>[7x]MTMFQYYKRSRHFVFSAFIAFVFVLLCQNTAFARASSNGDLPTKADLQAQLDSLNKQKDLSAQDKLVQQDLTDTLATLDKIDRIKEETVQLRQKVAEAPEKMRQATAALTALSDVDNDEETRKILSTLSLRQLETRVAQALDDLQNAQNDLASYNSQLVSLQTQPERVQNAMYNASQQLQQIRSRLDGTDVGETALRPSQKVLMQAQQALLNAEIDQQRKSLEGNTVLQDTLQKQRDYVTANSARLEHQLQLLQEAVNSKRLTLTEKTAQEAVSPDEAARIQANPLVKQELEINQQLSQRLITATENGNQLMQQNIKVKNWLERALQSERNIKEQIAVLKGSLLLSRILYQQQQTLPSADELENMTNRIADLRLEQFEVNQQRDALFQSDAFVNKLEEGHTNEVNSEVHDALLQVVDMRRELLDQLNKQLGNQLMMAINLQINQQQLMSVSKNLKSILTQQIFWVNSNRPMDWDWIKAFPQSLKDEFKSMKITVNWQKAWPAVFIAFLAGLPLLLIAGLIHWRLGWLKAYQQKLASAVGSLRNDSQLNTPKAILIDLIRALPVCLIILAVGLILLTMQLNISELLWSFSKKLAIFWLVFGLCWKVLEKNGVAVRHFGMPEQQTSHWRRQIVRISLALLPIHFWSVVAELSPLHLMDDVLGQAMIFFNLLLIAFLVWPMCRESWRDKESHTMRLVTITVLSIIPIALMVLTATGYFYTTLRLAGRWIETVYLVIIWNLLYQTVLRGLSVAARRIAWRRALARRQNLVKEGAEGAEPPEEPTIALEQVNQQTLRITMLLMFALFGVMFWAIWSDLITVFSYLDSITLWHYNGTEAGAAVVKNVTMGSLLFAIIASMVAWALIRNLPGLLEVLVLSRLNMRQGASYAITTILNYIIIAVGAMTVFGSLGVSWDKLQWLAAALSVGLSFGLQEIFGNFVSGLIILFERPVRIGDTVTIGSFSGTVSKIRIRATTITDFDRKEVIIPNKAFVTERLINWSLTDTTTRLVIRLGVAYGSDLEKVRKVLLKAATEHPRVMHEPMPEVFFTAFGASTLDHELRLYVRELRDRSRTVDELNRTIDQLCRENDINIAFNQLEVHLHNEKGDEVTEVKRDYKGDDPTPAVG

Amongst these family members, MscK is unique in that channel activation, in addition to elevated lateral membrane tension, requires the presence of certain external ions such as K+, Rb+, or Cs+ 32–34. The E. coli MscK (EcMscK) channel, consisting of 1120 amino acids, contains a large N-terminal periplasmic domain (PD, ~500 amino acids), a transmembrane domain (TMD) with eleven predicted TM helices, and a cytoplasmic domain (CTD) analogous to that of EcMscS. The MscK channel forms a symmetric heptamer, with each subunit comprised of three distinct layers: an N-terminal periplasmic PD, a TMD with eleven TM helices, and a C-terminal cytoplasmic CTD. To better understand the biophysical underpinnings of mechanotransduction and to establish the molecular basis of dual activation in a ligand- and force-gated channel, we have determined cryo-EM structures of EcMscK in distinct functional states by leveraging GOF mutants.

To potentially improve structural homogeneity and to achieve a functionally distinct conformation, we decided to characterize a GOF mutant G924S, which, in contrast to the WT channel, was active under elevated membrane tension in both KCl and NaCl conditions. Thus, the cryo-EM datasets of G924S in NaCl and in KCl were essentially indistinguishable, which allowed us to combine the datasets to further improve the reconstructions of both the closed and open conformations to overall resolutions of 3.84 and 3.47 Å, respectively. The final atomic models fit well into their respective densities and were refined to good stereochemistry. The lower resolution reconstruction of the WT channel is nearly identical to the closed conformation of G924S, and hereinafter the higher-resolution structures of G924S are primarily used for structural analysis and interpretation. The innermost pore-lining helix TM11 contains an apparent kink such that TM11a defines the transmembrane ion-conduction path and TM11b runs nearly parallel to the membrane plane and extends to the cytoplasmic CTD. Akin to EcMscS and AtMSL1, the pore-lining helix (TM11) in the resting state is kinked, and several bulky hydrophobic side chains point to the central pore axis to create narrow constrictions. A hydrophobic gate near the cytoplasm is constituted by V921 and F925, which are conserved amongst MscK homologs. In contrast to EcMscS and AtMSL1, an additional constriction at the periplasmic side of MscK, with a pore diameter of ~8 Å, is formed by a ring of seven tryptophan (W914) residues. It appears that MscK possesses two physically separated hydrophobic gates along the pore: an upper periplasmic gate and a lower cytoplasmic gate. The arrangement of the eleven TM helices generates a midplane bending angle of ~30°. The periplasmic gating ring is primarily held together by packing interactions of inter-subunit three-helix bundles, in which one of the interfacial helices engages its entirety at the interface in the closed conformation.>GSMELRVGNRYRLGRKIG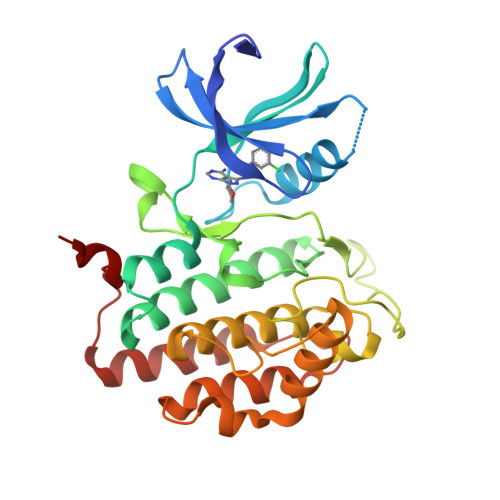SGSFGDIYLGTDIAAGEEVAIKLECVKTKHPQLHIESKIYKMMQGGVGIPTIRWCGAEGDYNVMVMELLGPSLEDLFNFCSRKFSLKTVLLLADQMISRIEYIHSKNFIHRDVKPDNFLMGLGKKGNLVYIIDFGLAKKYRDARTHQHIPYRENKNLTGTARYASINTHLGIEQSRRDDLESLGYVLMYFNLGSLPWQGLKAATKRQKYERISEKKMSTPIEVLCKGYPSEFATYLNFCRSLRFDDKPDYSYLRQLFRNLFHRQGFSYDYVFDWNMLK[2x]> MALPTPSDSTLPAEARGRGRRRRLVWTPSQSEALRACFERNPYPGIATRERLAQAIGIPEPRVQIWFQNERSRQLRQHRRESRPWPGRRGPPEGRRKRTAVTGSQTALLLRAFEKDRFPGIAAREELARETGLPESRI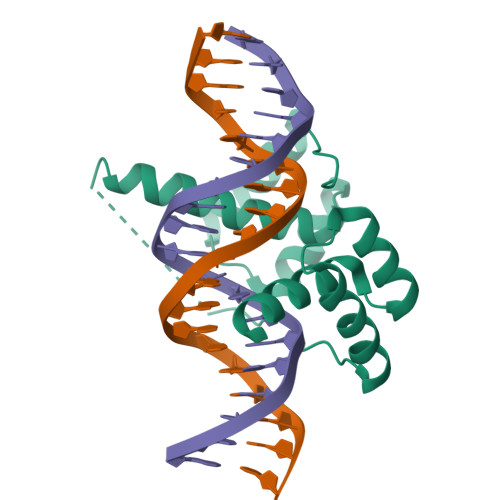QIWFQNRRARH> PELNKERPSLQIKLKIEDFILHKMLGKGSFGKVFLAEFKKTNQFFAIKALKKDVVLMD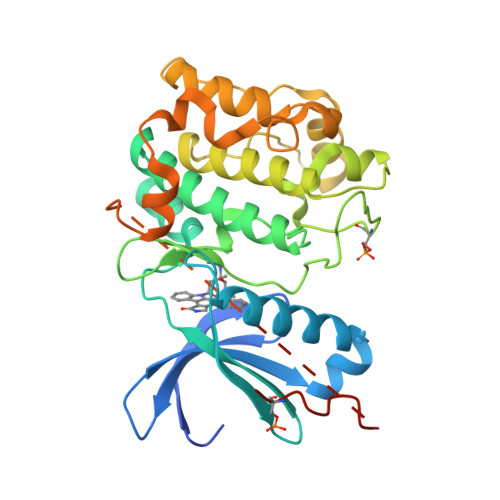DDVECTMVEKRVLSLAWEHPFLTHMFCTFQTKENLFFVMEYLNGGDLMYHIQSCHKFDLSRATFYAAEIILGLQFLHSKGIVYRDLKLDNILLDKDGHIKIADFGMCKENMLGDAKTNTFCGTPDYIAPEILLGQKYNHSVDWWSFGVLLYEMLIGQSPFHGQDEEELFHSIRMDNPFYPRWLEKEAKDLLVKLFVREPEKRLGVRGDIRQHPLFREINWEELERKEIDPPFRPKVKSPFDCSNFDKEFLNEKPRLSFADRALINSMDQNMFRNFSFMNPGMERLIS> SQIIRCKAAVAWEAGKPLVIEEVEVAPPQKHEVRIKILFTSLCHTDVYFWEAKGQTPLFPRIFGHEAGGIVESVGEGVTDLQPGDHVLPIFTGECGECRHCHSEESNMCDLLRINTERGGMIHDGESRFSINGKPIYHFLGTSTFSEYTVVHSGQVAKINPDAPLDKVCIVSCG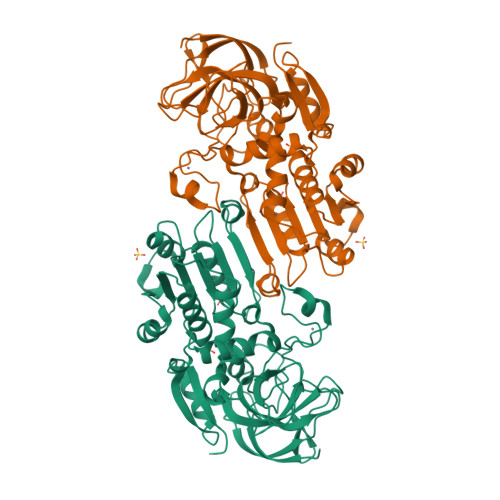LSTGLGATLNVAKPKKGQSVAIFGLGAVGLGAAEGARIAGASRIIGVDFNSKRFDQAKEFGVTECVNPKDHDKPIQQVIAEMTDGGVDRSVECTGSVQAMIQAFECVHDGWGVAVLVGVPSKDDAFKTHPMNFLNERTLKGTFFGNYKPKTDIPGVVEKYMNKELELEKFITHTVPFSEINKAFDYMLKGESIRCIITMGA> DRVYIHPFHLVIHNESTCEQLAKANAGKPKDPTFIPAPIQAKTSPVDEKALQDQLVLVAAKLDTEDKLRAAMVGMLANFLGFRIYGMHSELWGVVHGATVLSPTAVFGTLASLYLGALDHTADRLQAILGVPWKDKQCTSRLDAHKVLSALQAVQGLLVAQGRADSQAQLLLSTVVGVFTAPGLHLKQPFVQGLALYTPVVLPRSLDFTELDVAAEKIDRFMQAVTGWKTGSSLMGASVDSTLAFNTYVHFQGKMKGFSLLAEPQEFWVDQSTSVSVPMLSGMGTFQHWSDIQDQFSVTQVPFTESASLLLIQPHYASDLDKVEGLTFQQNSLNWMKKLSPRTIHLTMPQLVLQGSYDLQDLLAQAELPAILHTELNLQKLSNDRIRVGEVLNSIFFELEADEREPTESTQQLNKPEVLEVTLNRPFLFAVYDQSATALHFLGRVANPLSTAHHHHHH;> LTLGNTTSSVILTNYMDTQYYGEIGIGTPPQTFKVVFDTGSSNVWVPSSKCSRLYTACVYHKLFDASDSSSYKHNGTELTLRYSTGTVSGFLSQDIITVGGITVTQMFGEVTEMPALPFMLAEFDGVVGMGFIEQAIGRVTPIFDNIISQGVLKEDVFSFYYNRDSENSQSLGGQIVLGGSDPQHYEGNFHYINLIKTGVWQIQMKGVSVGSSTLLCEDGCLALVATGASYISGSTSSIEKLMEALGAKKRLFDYVVKCNEGPTLPDISFHLGGKEYTLTSADYVFQESYSSKKLCTLAIHAMDIPPPTGPTWALGATFIRKFYTEFDRRNNRIGFALAR

Human blood pressure is mainly controlled by the renin–angiotensin system, which consists of several key components, including renin, angiotensinogen (AGT),3 angiotensin-converting enzyme (ACE), and angiotensin receptors. Renin is a highly specific aspartic protease that cleaves AGT between Leu10 and Val11 to release the N-terminal angiotensin I peptide. Cleavage of AGT by renin is the rate-limiting step of the renin–angiotensin system. To address these questions, here we have solved high-resolution crystal structures of human glycosylated AGT, its encounter complex with renin, AGT cleaved in the reactive center loop, and the spent AGT from which the N-terminal angiotensin peptide has been removed by renin.

An inactive human renin variant (D226A) was also prepared from HEK293 cells for crystallizing the encounter complex of renin and AGT. The crystal structure of the AGT–renin complex shows that the N-terminal tail of AGT is docked in the substrate-binding pocket of renin. The total surface area buried in the interface between AGT and renin is more than 2100 Å2; interactions between the N-terminal peptide and the renin active site account for about 50% of the buried surface, whereas interactions between the bodies of AGT and renin account for the rest. The Asp38 of renin is hydrogen-bonded to the carbonyl oxygen of the scissile bond and to a water molecule that is also within hydrogen-bond distance to the other mutated aspartic acid. The N-flap of renin in the renin–AGT complex is in a relatively open conformation with the tip of the flap shifted by about 5 Å when compared with that seen in the renin–peptide complex. The substantial interactions between the bodies of the two molecules are mainly hydrophobic. Most unexpectedly, we have found that the N terminus of AGT emerges from the renin active cleft and pokes into a surface cavity surrounded by helix H, sheet B, and helix A of AGT. This cavity corresponds to the hormone-binding pocket seen in two other serpins, thyroxine-binding globulin (TBG) and cortisol-binding globulin (CBG). The entire helix H (residues 330–336) is unwound, with the shift of residues 333–337 opening up the pocket to accommodate the N-terminal tail and with Asn331 and Asn334 shifting to form key hydrogen bonds with the body of renin. AGT appears to have adopted a “tail-in-mouth” mechanism for interacting with renin, where insertion of its N terminus into the hormone-binding pocket helps to stabilize a new conformation that forms a complementary surface on AGT for renin binding.>MEKQNIAVILARQNSKGLPLKNLRKMNGISLLGHTINAAISSKCFDRIIVSTDGGLIAEEAKNFGVEVVLRPAELASDTASSISGVIHALETIGSNSGTVTLLQPTSPLRTGAHIREAFSLFDEKIKGSVVSACPMEHHPLKTLLQINNGEYAPMRHLSDLEQPRQQLPQAFRPNGAI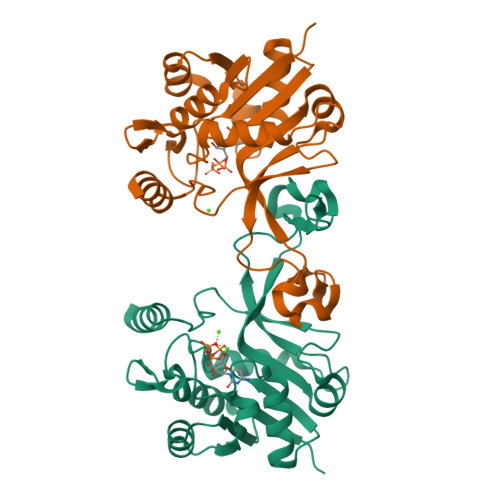YINDTASLIANNCFFIAPTKLYIMSHQDSIDIDTELDLQQAENILNHKES[2x]> AANDNNVEWNGLFHDQGPLFDNAPEPTSTQSVTLKLRTFKGDITSANIKYWDTADNAFHWVPMVWDSNDPTGTFDYWKGTIPASPSIKYYRFQINDGTSTAWYNGNGPSSTEPNADDFYIIPNFKTPDWLKNGVMYQIFPDRFYNGDSSNDVQTGSYTYNGTPTEKKAWGSSVYADPGYDNSLVFFGGDLAGIDQKLGYIKKTLGANILYLNPIFKAPTNHKYDTQDYMAVDPAFGDNSTLQTLINDIHSTANGPKGYLILDGVFNHTGDSHPWFDKYNNFSSQGAYESQSSPWYNYYTFYTWPDSYASFLGFNSLPKLNYGNSGSAVRGVIYNNSNSVAKTYLNPPYSVDGWRLDAAQYVDANGNNGSDVTNHQIWSEFRNAVKGVNSNAAIIGEYWGNANPWTAQGNQWDAATNFDGFTQPVSEWITGKDYQNNSASISTTQFDSWLRGTRANYPTNVQQSMMNFLSNHDITRFATRSGGDLWKTYLALIFQMTYVGTPTIYYGDEYGMQGGADPDNRRSFDWSQATPSNSAVALTQKLITIRNQYPALRTGSFMTLITDDTNKIYSYGRFDNVNRIAVVLNNDSVSHTVNVPVWQLSMPNGSTV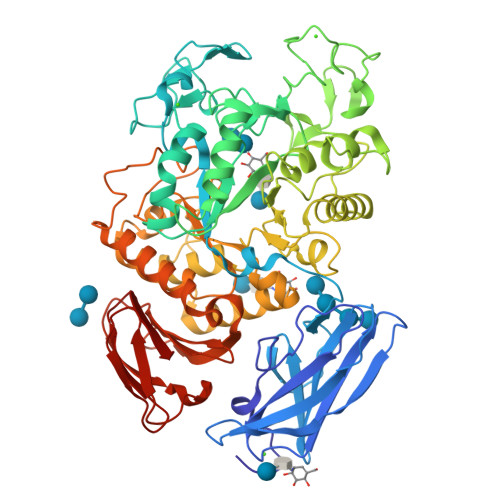TDKITGHSYTVQNGMVTVAVDGHYGAVLAQ> MSQFFYIHPDNPQQRLINQAVEIVRKGGVIVYPTDSGYALGCKIEDKNAMERICRIRQLPDGHNFTLMCRDLSELSTYSFVDNVAFRLMKNNTPGNYTFILKGTKEVPRRLLQEKRKTIGMRVPSNPIAQALLEALGEPMLSTSLMLPGSEFTESDPEEIKDRLE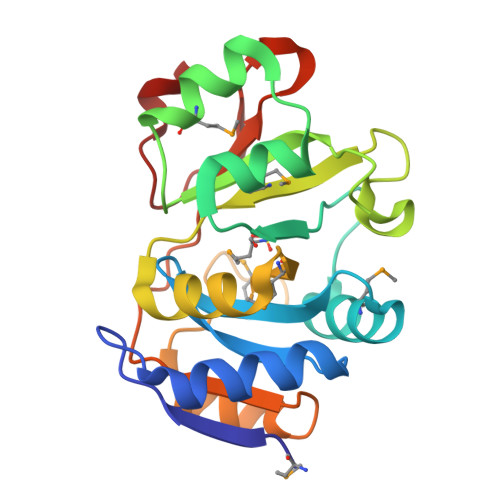KQVDLIIHGGYLGQKPTTVIDLTDDTPVVVREGVGDVKPFL> MDINIDDILAELDKETTAVDSTKITQGSSSTTHRDANTIVGSSLDLNDKTQIYVSPQQDFSDLMKSWKNERCSPELLPYPHQLMKRLLNRISMQSQLIENISMGFLDMQNASNANPPMPNESKLPLLCMETELERLKFVIRSYIRCRLSKIDKFSLYLRQLNEDENSLISLTDLLSKD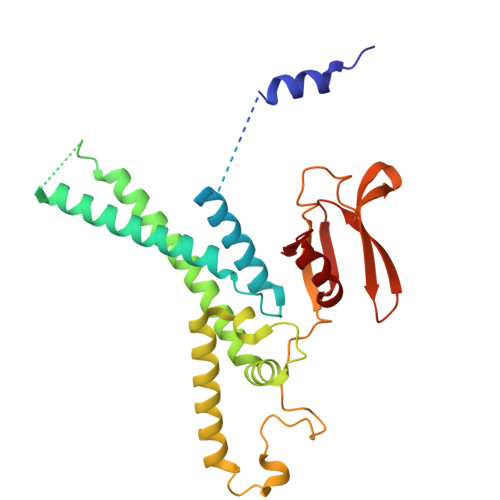EIKYHDTHSLIWLKLVNDSILKYMPEELQAINDTEGSVNMIDEPDWNKFVFIHVNGPPDGKWNEDPLLQENEFGKPCYTVTIPDLKEEVELTIGSIYVMRYEVIRDLLRDDKVALI>MKYLLPTAAAGLLLLAAQPAMAMATDHSPTVETRAAADNGTVKLGYFTEWGTYDRNFNVKNLDTSGTAAKITHINYAFGNVTGGKCAIGDSYADYDKAFTADQSVSGQADTWDQPLRGNFNQLRQLKAKYPHIKVLWSFGGWTWSGGFADAAKDPQGFAQSCYNLVHDPRWDGVFDGIDIDWEYPNACGLTCDSSGPDAFRNLMAALRSTFGDELVTAAVTADGTPGGKIEATDYAGAAQYVDWYNVMTYDFFGAWDAQGPTAPHSPLTSYDGIPKQGFTSADAIAAFKAQGVPADKLLLGIGFYGRGWTGVTQDAPGGTATGPAAGTWEQGIEDYKVLKNTCPVTGTVAGTAYAHCGSNLWSYDTP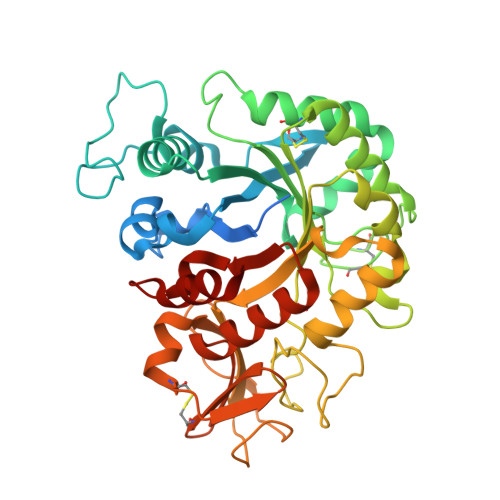DTIASKMAWANDQGLRGAFAWDFSGDTADGELIAALSNGLA[2x]4-phenylpyrimidine | C10 H8 N2 | 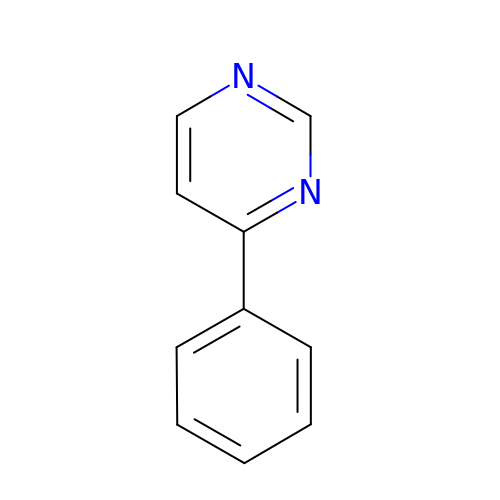MKLQPIYLZMLAER-UHFFFAOYSA-N> ADTIVAVELDTYPNTDIGDPNYQHIGINIKSIRSKATTRWNVQDGKVGTAHISYNSVAKRLSAIVSYPGGSSATVSYDVDLNNILPEWVRVGLSASTGVYKET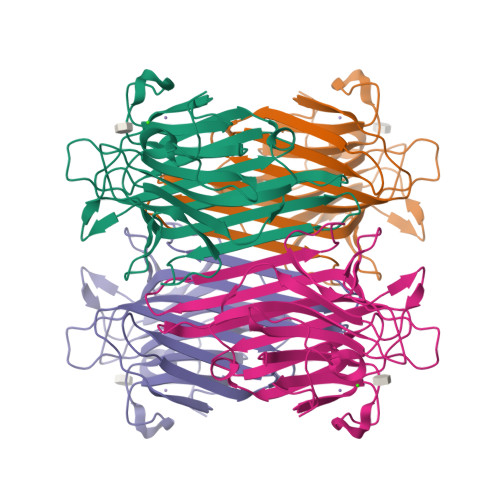NTILSWSFTSKLKTNSTADAQSLHFTFNQFSQSPKDLILQGDASTDSDGNLQLTRVSNGSPQSNSVGRALYYAPVHVWDKSAVVASFDATFTFLIKSPDSDPADGIAFFIANTDSSIPHGSGGRLLGLFPDAN The human RNA helicase DDX1 in the DEAD-box family plays an important role in RNA processing and has been associated with HIV-1 replication and tumour progression. DDX1 differs from all other DEAD-box proteins in a novel structural feature, a SPRY insertion domain in the helicase core. In DDX1, this DEAD-box core fold is disrupted by the large SPRY domain, prominently positioned in RecA-like domain 1 between the P-loop (Walker A) motif and conserved motif Ia (Godbout et al., 1994), which separates the motifs by around 240 residues instead of the usual to 20–40 residues as in other DEAD-box proteins. SPRY domains are known to function as protein–protein interaction platforms.

The protein construct used in the final crystallization setup consisted of residues 72–283 of human DDX1; however, clear electron density was only observed for residues 86–275 of chain A and residues 86–279 of chain B. The residues at the N- and C-terminus that could not be modelled are likely to be disordered in the crystal since we observed some ambiguous density that could not be interpreted. The models for the polypeptide chains A and B have a Cα r.m.s. deviation of 0.256 Å for alignment of all 193 residues (an r.m.s. deviation of 1.239 Å for all atoms), indicating that they are almost identical. hDSPRY adopts a compact β-sandwich conformation. The β-sandwich fold is slightly twisted and forms a bowl-like platform. Two layers of concave β-sheets stack together and are referred to in the following as β-sheets 1 and 2, and a third small β-sheet covers one side of the β-sandwich. β-Sheet 1 is composed of eight strands (β16, β1, β4, β13, β7, β8, β9 and β10), β-sheet 2 is composed of six strands (β2, β3, β14, β6, β11 and β12) and the small β-sheet 3 consists of only two strands (β15 and β5). We have discovered a positively charged surface region in hDSPRY that is highly conserved in DDX1 across species. This surface patch might constitute the protein–protein interaction site within hDSPRY.

>[2x]GSQEGKKGKTTIKTGASVLNKWQMNPYDRGSAFAIGSDGLCCQSREVKEWHGCRATKGLMKGKHYYEVSCHDQGLCRVGWSTMQASLDLGTDKFGFGFGGTGKKSHNKQFDNYGEEFTMHDTIGCYLDIDKGHVKFSKNGKDLGLAFEIPPHMKNQALFPACVLKNAELKFNFGEEEFKFPPKDGFVALSKAPDGYIVKSQHSGNAQVTQTKFLEHHHHHH> KTSCLMATGVLKCPTDPEAVKKVHIDLWDAAAAAAESDDLMGRTWSDRNGNFQVTGCASDFGPINTPDPYLYIQHNCPHRDSNATNPIQIDVIPLFLPSIVRLGNVYLDRYL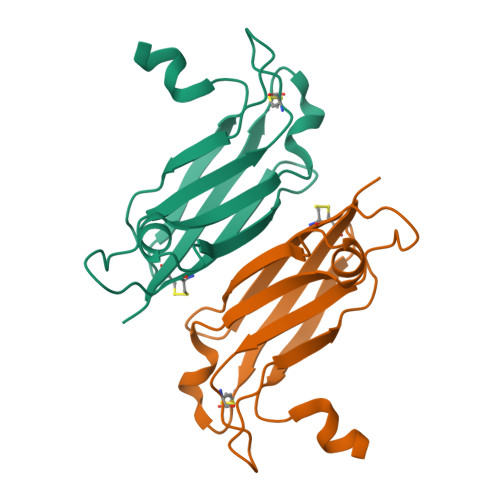EDYHH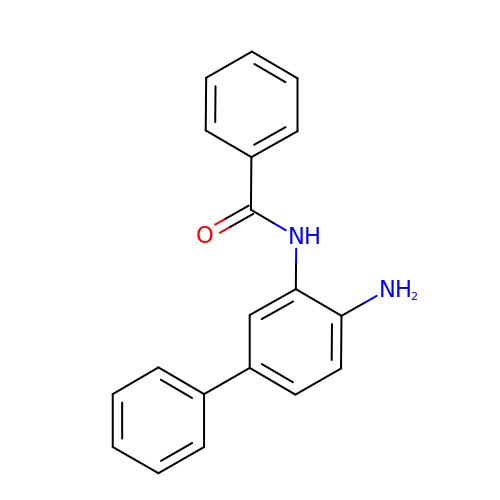N-(4-aminobiphenyl-3-yl)benzamide | C19 H16 N2 O | ZWLFHHHQRUYIBT-UHFFFAOYSA-N>[2x]G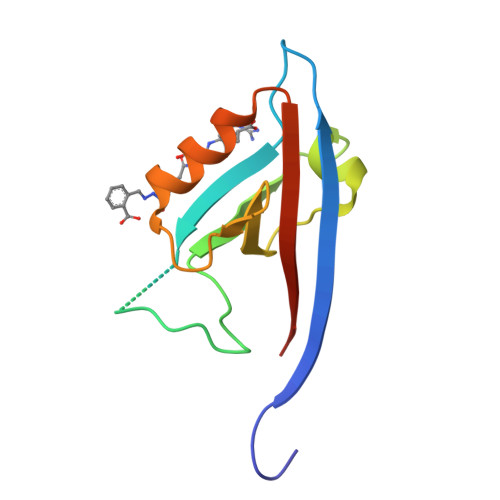PLGSDYIIKEKTVLLQKKDSEGFGFVLRGAKAQTPIEEFTPTPAFPALQYLESVDEGGVAWRAGLRMGDFLIEVNGQNVVKVGHRQVVNMIRQGGNTLMVKVVMVTRHPDM> SADKVESLDVDSEAKKLLGLGQKHLVMGDIPAAVNAFQEAASLLGKKYGETANECGEAFFFYGKSLLELARLENKSLQENEEEEIGNLELAWDMLDLAKIIFKRQETKEAQLYAAQAHLKLGEVSVESENYVQAVEEFQSCLNLQEQYLEAHDRLLAETHYQLGLAYGYNSQYDEAVAQFSKSIEVIENRMAVLNEQVKEAEGSSAEYKKEIEELKELLPEIREKIEDAKESQRSGNVAELALKATLVESST

NASP is a major histone chaperone for H3–H4 dimers critical for preventing histone degradation. NASP and its homologues share an atypical tetratricopeptide repeat (TPR) domain. They constitute the SHNi-TPR (Sim3-Hif1-NASP interrupted TPR) family, predicted to have four TPR motifs with the TPR2 motif being interrupted by a long acidic region, a capping helix region immediately following the TPR4 motif, and a disordered C-terminal region containing a nuclear localization signal (NLS). Here, we report the crystal structures of the sNASP dimer, the complex of sNASP with an H3 α3 peptide, and the sNASP–H3–H4–ASF1b co-chaperone complex.

To facilitate crystallization, we made a construct containing the TPR domain and capping helix region of human sNASP with the acidic region deleted (a.a 30–340 with a deletion Δ101–159; hereafter referred to as ‘sNASP core’, sNASPc). During gel-filtration purification, sNASPc was shown to have two peaks (conformations) on the chromatogram. The two protomers in the structure are related by a 2-fold symmetric axis with each protomer containing four TPR motifs. The extended α89 is constituted of residues from Tyr261 to Gly324 (64-residues long) of sNASPc with a kink at Glu305, and the kinked α89 helix is totally about 95 Å (65 Å + 30 Å) in length. The α89 and α89′ twist one another in a left-handed manner to form an antiparallel coiled-coil like structure, with the C-terminal one third of α89′of the sNASPc’ protomer further packing against α7 and the N-terminal one third of α89 of the sNASPc protomer, and vice versa. Thus, the C-terminal one third of the α89 and α89′ helices each function like a ‘capping helix’, forming the unique architecture of a domain-swapping and dumbbell-shape dimer. The coiled-coil like interactions between α89 and α89′ constitute of totally 66 residues (33 residues from each helix), of which the predominant interactions are hydrophobic interactions and van der Waals contacts, with a few hydrogen bonds and salt bridges further stabilizing the dimer. Consistent with the extensive interactions, many different mutants with single or even double mutations along the dimer interface failed to disrupt the dimer, and only a mutant with substitutions of six hydrophobic residues by glutamate (V265E I272E L282E V286E I300E L307E; Hereafter referred to as 6E mutant) was found to abolish the dimer formation. The purified sNASPc dimer at a concentration of 5 mg/ml was crystallized in 0.2 M Calcium acetate, 0.1 M HEPES, pH 7.5, 40% v/v PEG 400, with the sitting-drop vapor-diffusion method at 20°C. The concentration of PEG 400 in the mother liquor was high enough to serve as cryoprotectant, thus all crystals were directly flash frozen in liquid nitrogen.> 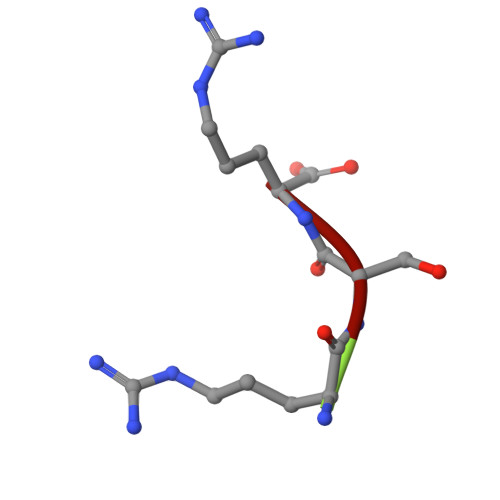RSR>[2x]AGENLYFQSLMNNFGNEEFDCHF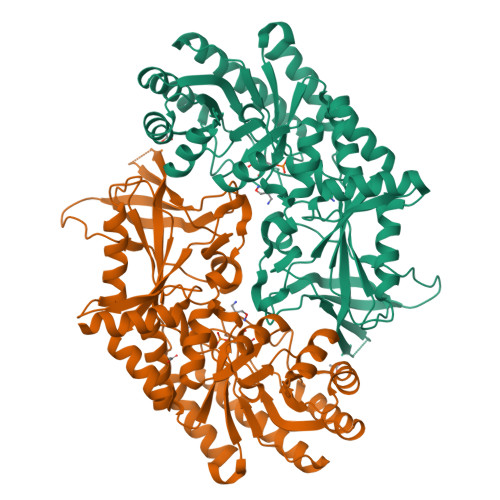LDEGFTAKDILDQKINEVSSSDDKDAFYVADLGDILKKHLRWLKALPRVTPFYAVKCNDSKAIVKTLAATGTGFDCASKTEIQLVQSLGVPPERIIYANPCKQVSQIKYAANNGVQMMTFDSEVELMKVARAHPKAKLVLRIATDDSKAVCRLSVKFGATLRTSRLLLERAKELNIDVVGVSFHVGSGCTDPETFVQAISDARCVFDMGAEVGFSMYLLDIGGGFPGSEDVKLKFEEITGVINPALDKYFPSDSGVRIIAEPGRYYVASAFTLAVNIIAKKIVLKEQTGSDDEDESSEQTFMYYVNDGVYGSFNCILYDHAHVKPLLQKRPKPDEKYYSSSIWGPTCDGLDRIVERCDLPEMHVGDWMLFENMGAYTVAAASTFNGFQRPTIYYVMSGPAWQLMQQFQNPDFPPEVEEQDASTLPVSCAWESGMKRHRAACASASINV> SCPAIHVFGARETTASPGYGSSSTVVNGVLSAYPGSTAEAINYPACGG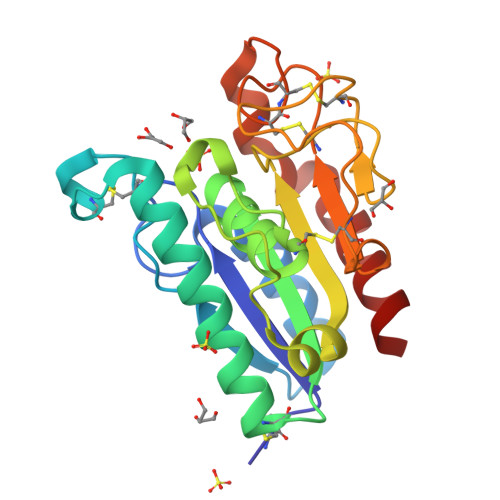QSSCGGASYSSSVAQGIAAVASAVNSFNSQCPSTKIVLVGYSQGGEIMDVALCGGGDPNQGYTNTAVQLSSSAVNMVKAAIFMGDPMFRAGLSYEVGTCAAGGFDQRPAGFSCPSAAKIKSYCDASDPYCCNGSNAATHQGYGSEYGSQALAFVKSKLG> ALPQTVRIGTDTTYAPFSSKDAKGEFIGFDIDLGNEMCKRMQVKCTWVASDFDALIPSLKAKKIDAIISSLSITDKRQQEIAFSDK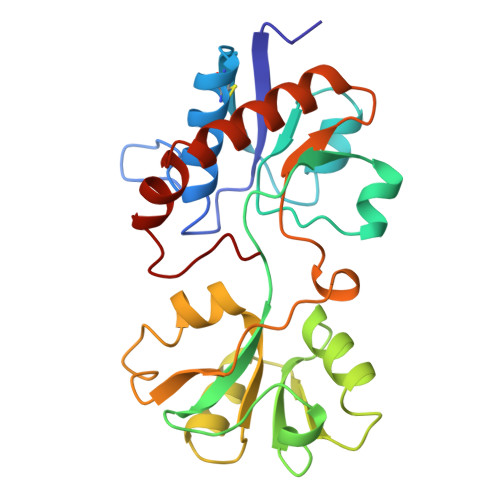LYAADSRLIAAKGSPIQPTLESLKGKHVGVLQGSTQEAYANDNWRTKGVDVVAYANQDLIYSDLTAGRLDAALQDEVAASEGFLKQPAGKEYAFAGPSVKDKKYFGDGTGVGLRKDDTELKAAFDKALTELRQDGTYDKMAKKYFDFNVYGD> MANTDYAGNLTRPHWGGAASDVDIHLEVYQNEVDTRFQYQAMFLGLSSQRSVADRSNTYRIDRLNTSSVKGRTSGVALEPTPVRNDKMLIVVDTVLYIRNPIDYQDDWTAPDFLTEMGQNNGSEFAEVFDQAHLIQLIKGRSWVAPAHLKPAFSDGIEIEATIDSDVTTQAGMEANAIAINQAHKAGIDELIKRKVPLNDMITLVSTEIYSLLLEHPKLFNKDWG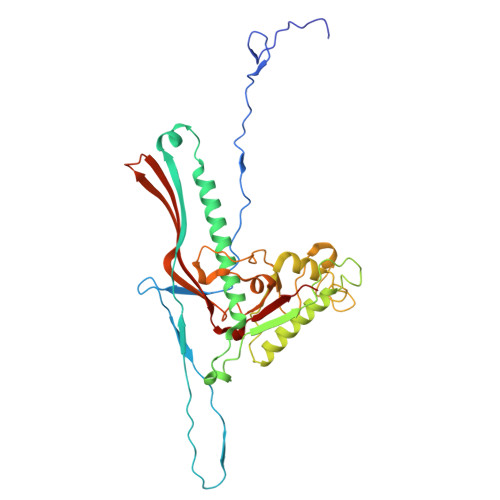DANANGYKERRAVLMNGIPVVECTEFPDAGTHPLGSAYTVTADDAKCRMVTFSKSRTLVTVEAKPFTSRIWDDEQNFANVLDCYAMYQVGERRPDTAAVVKFNEAP>[2x]GSLAEVLAETVRWLRLAREDPEAFAARVAALLADPDAFSPTEVAAAYVALAVLAR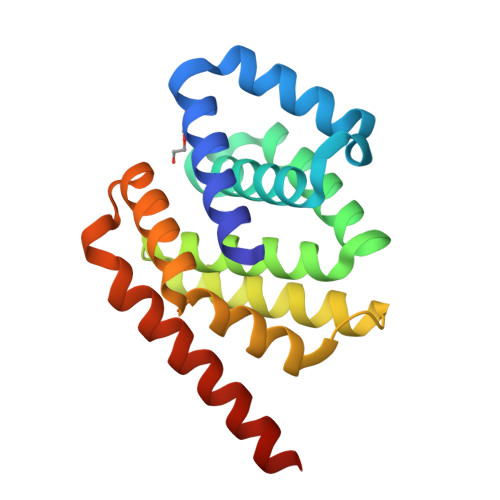ERGDAEAAAAAERLGAHLLATDPETYLEAQVVLAAIEALLGREEEAEAVLEEALSRLTAANKGDKKDLLKAIKKLFEPEARAQLAAIAAVLDAADNVEAALARLEKWAERLEKELEHHHHHH> MQIYSEYYEKIGPRKLRLLVKRRLLFASTWLYINNYI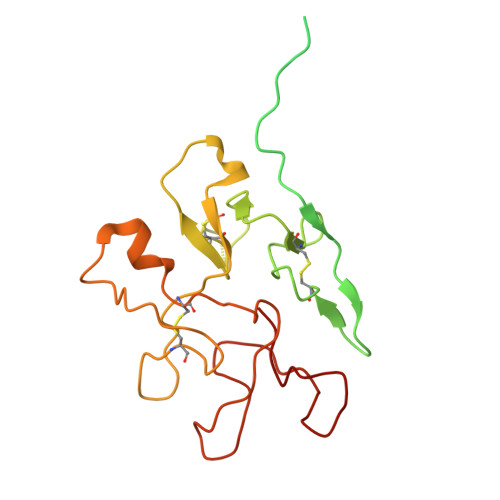LLSIIMKLQTKHMILLGFVAVVVVFIIFMLTRKKKEGFSIGNIFGKVKGAVTGTVGKVVNVVKPQGYKPEFVNRVNFGKFWACPEGTTDWGSEDKQCLVSQYGPMMWRNKGGNEWGWSCPAGSAPNNSDDWNQKCVQGYSMKKLIDGQWRCTDTEIDTGKDWSNSDWFTAQQQCDRGNNKVFTRRMYIDGKWQCPDGTWDTGFTWSDGENGGKQCKYYP> THVDLGLASANVDFAFSLYKQLVLKAPDKNVIFSPLSISTALAFLSLGAHNTTLTEILKGLKFNLTETSEAEIHQSFQHLLRTLNQSSDELQLSMGNAMFVKEQL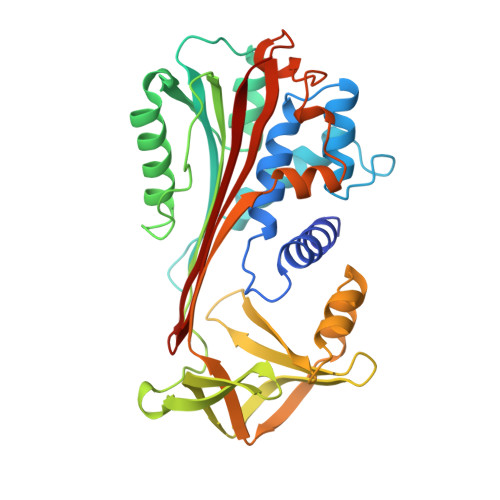SLLDRFTEDAKRLYGSEAFATDFQDSAAAKKLINDYVKNGTRGKITDLIKDLDSQTMMVLVNYIFFKAKWEMPFDPQDTHQSRFYLSKKKWVMVPMMSLHHLTIPYFRDEELSCTVVELKYTGNASALFILPDQDKMEEVEAMLLPETLKRWRDSLEFREIGELYLPKFSISRDYNLNDILLQLGIEEAFTSKADLSGITGARNLAVSQVVHKAVLDVFEEGREASAATAVKITLL>[2x]MGHHHHHHEFMTSRPSSDQT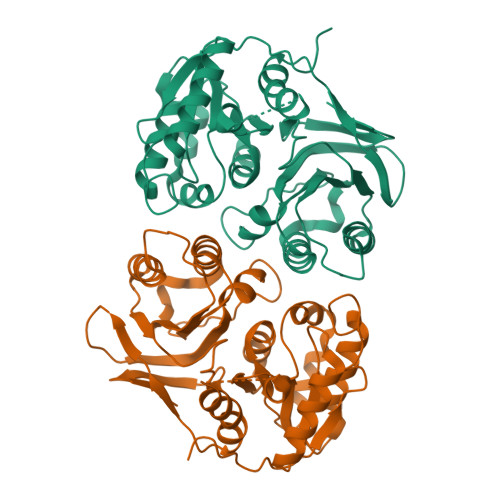WQPIDGRVALIAPASAIATEVLEATLRQLEVHGVDYHLGRHVEARYRYLAGTVEQRLEDLHNAFDMPDITAVWCLRGGYGCGQLLPGLDWGRLEAASPRPLIGFSDISVLLSAFHRHGLPAIHGPVATGLGLSPLSAPREQQERLASLASVSRLLAGIDHELPVQHLGGHKQRVEGALIGGNLTALACMAGTLGGLHAPAGSILVLEDVGEPYYRLERSLWQLLESIDARQLGAICLGSFTDCPRKEVAHSLERIFGEYAAAIEVPLYHHLPSGAGAQNRAWPYGKTAVLEGNRLRW TFIIB-related factor 2 (Brf2) is a member of the family of TFIIB-like core transcription factors. Brf2 recruits RNA polymerase (Pol) III to type III gene-external promoters, including the U6 spliceosomal RNA and selenocysteine tRNA genes. We have solved crystal structures of a human Brf2-TBP complex bound to natural promoters, obtaining a detailed view of the molecular interactions occurring at Brf2-dependent Pol III promoters and highlighting the general structural and functional conservation of human Pol II and Pol III pre-initiation complexes. Surprisingly, our structural and functional studies unravel a Brf2 redox-sensing module capable of specifically regulating Pol III transcriptional output in living cells.

We obtained X-ray crystallographic structures of Brf2-TBP complexes bound to the U6 snRNA (copy number 2, U6-2), RPPH1, and TRNAU1 promoters at resolutions of 1.9 Å, 2.2 Å, and 2.7 Å, respectively. Where not stated otherwise, we focus on the analysis of the complex solved at the highest resolution, the Brf2-TBP/U6-2 complex (hereafter referred to as the Brf2-TBP/DNA complex), but the conclusions apply to all three complexes. The overall architecture of the Brf2-TBP/DNA complex is reminiscent of the TFIIB-TBP/DNA complex (Nikolov et al., 1995, Tsai and Sigler, 2000), thus providing experimental support to the proposed common architectural organization of TFIIB-related factors and TFIIB. Brf2 contacts extensively the phosphate backbone of the DNA and establishes sequence-specific contacts with both the upstream and downstream TATA flanking regions. The highly conserved dyad K113 and K114 contacts the phosphate backbone of the DNA on opposite sides, allowing the insertion of a short helix into the minor groove and the consequent direct recognition of bases A+3 and G′+4 (numbering is relative to the edge of the TATA box, with the non-template strand designated by a prime). The side chain of R110 forms a direct hydrogen bond with A+3 and a water-mediated hydrogen bond with G′+4, whereas the main chain carbonyl oxygen of A108 forms a direct hydrogen bond with G′+4. These interactions locally distort the DNA, leaving the base T′+3 unstacked at its downstream edge. Brf2 residue Y260 establishes a hydrogen bond and a T-shaped π-π interaction with nucleobase C−4 and an additional T-shaped π-π interaction with nucleobase C−3. A Brf2-specific short structured element (residues 357–363), the “molecular pin,” encompasses a conserved LPPC motif and lies at the ternary interface between the Brf2 C-terminal cyclin repeat, TBP, and the DNA. At the tip of the molecular pin, the Brf2 residue C361 is buried in the groove between two adjacent phosphate groups of the DNA backbone, establishing both van der Waals and water-mediated hydrogen bonds at the upstream edge of the TATA box.

> GPNEQVSRSQQRGLRRVRDLCRVLQLPPTFEDTAVAYYQQAYRHSGIRAARLQKKEVLVGCCVLITCRQHNWPLTMGAICTLLYADLDVFSSTYMQIVKLLGLDVPSLCLAELVKTYCSSFKLFQASPSVPAKYVEDKEKMLSRTMQLVELANETWLVTGRHPLPVITAATFLAWQSLQPADRLSCSLARFCKLANVDLPYPASSRLQELLAVLLRMAEQLAWLRVLRLDKRSVVKHIGDLLQHRQSLVRSAFRDGTAEVETREKEPPGWGQGQGEGEVGNNSLGLPQGKRPASPALLLPPCMLKSPKRICPVPPVSTVTGDENISDSEIEQYLRTPQEVRDFQRAQAARQAATSVPNPP;> GPSGIVPQLQNIVSTVNLGCKLDLKTIALRARNAEYNPKRFAAVIMRIREPRTTALIFSSGKMVCTGAKSEEQSRLAARKYARVVQKLGFPAKFLDFKIQNMVGSCDVKFPIRLEGLVLTHQQFSSYEPELFPGLIYRMIKPRIVLLIFVSGKVVLTGAKVRAEIYEAFENIYPILKGFRKTT> HHHHHHPEIVDTCSLASPASVCRTKHLHLRCSVDFTRRTLTGTAALTVQSQEDNLRSLVLDTKDLTIEKVVINGQEVKYALGERQSYKGSPMEISLPIALSKNQEIVIEISFETSPKSSALQWLTPEQTSGKEHPYLFSQCQAIHCRAILPCQDTPSVKLTYTAEVSVPKELVALMSAIRDGETPDPEDPSRKIYKFIQKVPIPCYLIALVVGALESRQIGPRTLVWSEKEQVEKSAYEFSETESMLKIAEDLGGPYVWGQYDLLVLPPSFPYGGMENPCLTFVTPTLLAGDKSLSNVIAHEISHSWTGNLVTNKTWDHFWLNEGHTVYLERHICGRLFGEKFRHFNALGGWGELQNSVKTFGETHPFTKLVVDLTD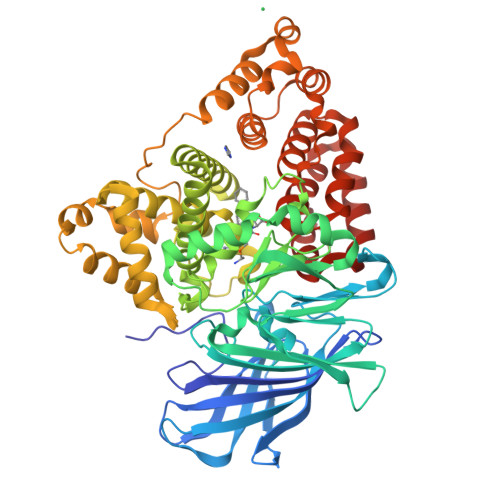IDPDVAYSSVPYEKGFALLFYLEQLLGGPEIFLGFLKAYVEKFSYKSITTDDWKDFLYSYFKDKVDVLNQVDWNAWLYSPGLPPIKPNYDMTLTNACIALSQRWITAKEDDLNSFNATDLKDLSSHQLNEFLAQTLQRAPLPLGHIKRMQEVYNFNAINNSEIRFRWLRLCIQSKWEDAIPLALKMATEQGRMKFTRPLFKDLAAFDKSHDQAVRTYQEHKASMHPVTAMLVGKDLKVD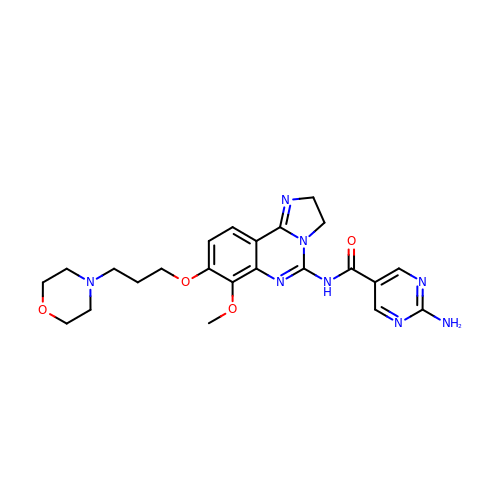2-azanyl-~{N}-[7-methoxy-8-(3-morpholin-4-ylpropoxy)-2,3-dihydroimidazo[1,2-c]quinazolin-5-yl]pyrimidine-5-carboxamide | C23 H28 N8 O4 | PZBCKZWLPGJMAO-UHFFFAOYSA-N> MIEPSVEEFPAENGPQLTPELAIANLQSSDL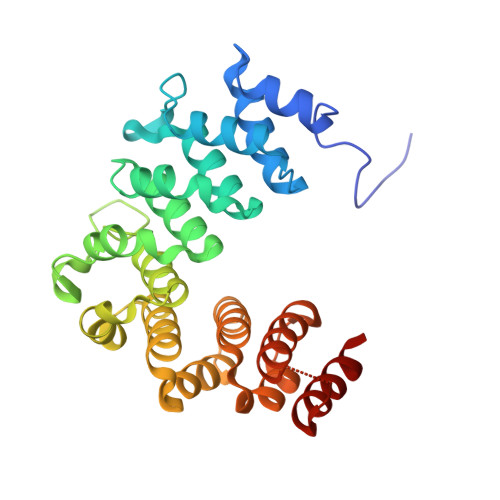SLRYYAAWWLGKYRVKESAAVDALIAALEDEADRTELGGYPLRRNAARALGKLGNRKAVPGLINCLECPDFYVREAAAQSLEMLKDKTAAPALIKLLDGGVAQAVQVTGRPHLVQPYEAVLEALGAIGATDAIPLIQPFLEHPVSRVQCAAARAMYQLTQEPVYGELLVKVLAGNDLNLRRVALGDLGAIGYLAAAEAIANAKAENSFKLIALKGLLEHQMSAESNALSISDQAIRVMNLMDSLL> DFSTIPIDYVKAKDPNTIDFCLSYLELYHTTKAVKACTPFSFILGSDAGMQRATETTES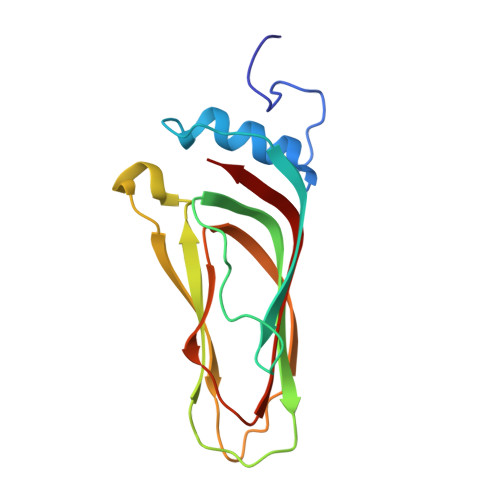LYWGKVILDINPNLSPLVNTTIVLEIESMLSSNSINRSENKRITRYIEKENFVNESSERFEFFKSMELSHLSTAYDVYVTFIGFKIDL>MQHLVLIGFMGSGKSSLAQELGLALKLEVLDTDMIISE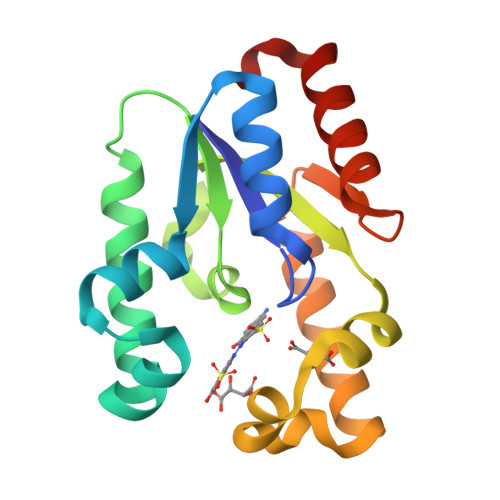RVGLSVREIFEELGEDNFRMFEKNLIDELKTLKTPHVISTGGGIVMHENLKGLGTTFYLKMDFETLIKRLNQKERAKRPLLNNLTQAKELFEKRQALYEKNASFIIDARGGLNNSLKQVLQFIALQPSLS[3x]> MELGESFLMPYSLEEQT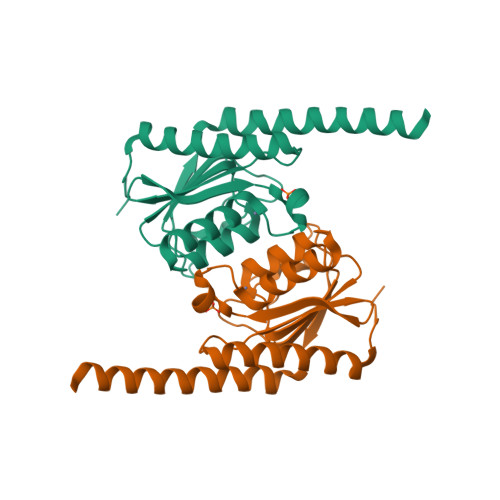YFMQEALKESEKSLQKAEIPIGCVIVKDGEIIGRGHNAREESNQAIMHAEMMAINEANAHEGNWRLLDTTLFVTIEPCVMCSGAIGLARIPHVIYGASNQKFGGVDSLYQILTDERLNHRVQVERGLLAADCANIMQTFFRQGRERKKIAKHLIKEQSDPFD> GSNRRLQQTQAQVDEVVDIMRVNVDKVLERD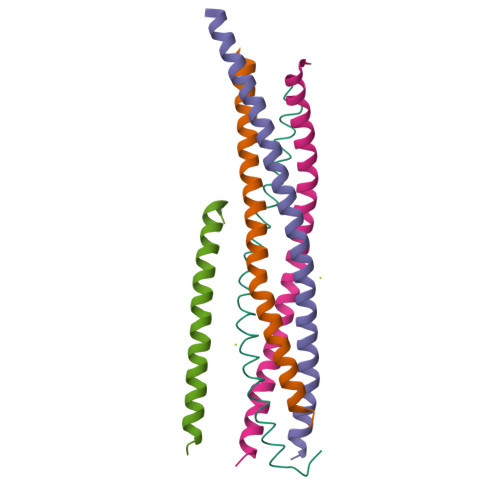QKLSELDDRADALQAGASQFETSAAKLKRKYWWKN;> GSALSEIETRHSEIIKLENSIRELHDMFMDMAMLVESQGEMIDRIEYNVEHAVDYVERAVSD;> GSLEEMQRRADQLADESLESTRRMLQLVEESKDAGIRTLVMLDEQGEQLDRVEEGMNHINQDMKEAEKNLKDLW;> GSARENEMDENLEQVSGIIGNLRHMALDMGNEIDTQNRQIDRIMEKADSNKTRIDEANQRATKMLW;> GSKDPDAAKKEEERQEALRQAEEERKAKYAKMEAEREVMRQGIRDKYGI>MGRRRSHERRDLPPNLYIRNNGYYCYRDPRTGKEFGLGRDRRIAITEAIQANIELFSGHKHKPLTARINSDNSVTLHSWLDRYEKILASRGIKQKTLINYMSKIKAIRRGLPDAPLEDITTKEIAAMLNGYIDEGKAASAKLIRSTLSDAFREAIAEGHITTNHVAATRAAKSKVRRSRLTADEYLKIYQAAESSPCWLRLAMELAVVTGQRVGDLCEMKWSDIVDGYLYVEQSKTGVKIAIPTALHIDALGISMKETLDKCK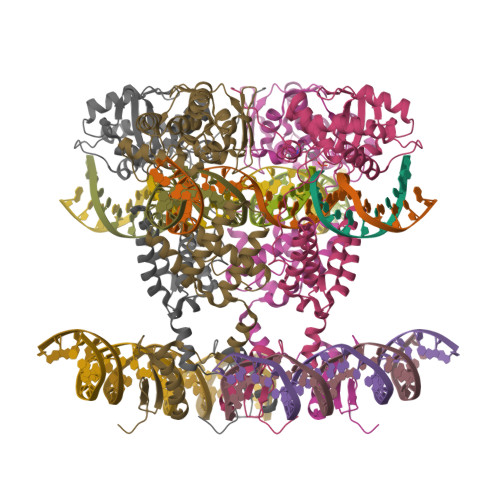EILGGETIIASTRREPLSSGTVSRYFMRARKASGLSFEGDPPTFHELRSLSARLYEKQISDKFAQHLLGHKSDTMASQYRDDRGREWDKIEIK[2x]Phytochromes are biliprotein photoreceptors widespread amongst microorganisms and ubiquitous in plants where they control developmental processes as diverse as germination, stem elongation and floral induction through the photoconversion of inactive Pr to the Pfr signalling state. The principal role of phyA is to detect exceedingly low light levels by integrating photons over prolonged periods, whereby molecules in the inactive Pr state are converted to and accumulate as the Pfr signalling state in the nucleus (the very low fluence response or VLFR). Here we report crystal structures of the chromophore-binding module of soybean phytochrome A, including ~2.2 Å XFEL structures of Pr and Pfr at ambient temperature and high resolution cryogenic structures of Pr. Here we present several novel 3D structures of a minimal soybean phyA(nPAS-GAF) construct as Pr and Pfr.

Phytochromobilin (PΦB) rather than PCB is the native chromophore in plant phytochromes. Indeed, the different adducts show subtle differences: not only is λmax red-shifted on account of the PΦB D-ring vinyl side chain, in phyB, the rate of thermal reversion in vitro is faster for PΦB- than for PCB-adducts. In the case of the present phyA construct, the thermal reversion half-lives of the PCB and PΦB adducts were 112 and 55 min, respectively. Apparent differences in water mobilities might provide a clue (see Supplementary Discussion).

>[2x]MISGTADGVNQPRHDKVTTAYLHHMQKGKMIQPFGCLLALDEKTCKVIAYSENAPEMLTMVSHAVPSVGDHPALGIGTDIKTLFTAPSASALQKALGFAEVLLLNPVLIHCKTSGKPFYAIIHRVTGSMIIDFEPVKPYEVPMTAAGALQSYKLAAKAITRLQSLPSGSMERLCDTMVQEVFELTGYDRVMAYKFHEDDHGEVIAEITKPGLEPYLGLHYPATDIPQASRFLFMKNKVRMIVDCHAKHVRVLQDEKLPFDLTLCGSTLRAPHSCHAQYMANMDSIASLVMAVVVNDNEEDGDTDAIQPQKRKRLWGLVVCHNTTPRFVPFPLRYACEFLAQVFAIHVNKEIELHHHHHH> MTSFQEVPLQTSNFAHVIFQNVAKSYLPNAHL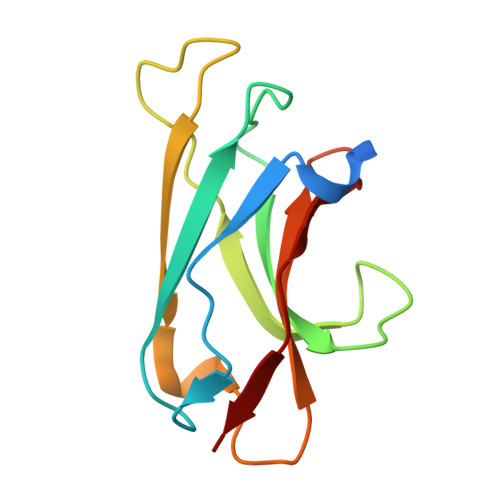ECHYTLTPYIHPHPKDWVGIFKVGWSTARDYYTFLWSPMPEHYVEGSTVNCVLAFQGYYLPNDDGEFYQFCYVTHKGEIRGASTPFQFR> MESKKRQWALEDFEIGRPLGKGKFGNVYLAREKQSKFILALKVLFKAQLEKAGVEHQLRREVEIQSHLRHPNILRLYGYFHDATRVYLILEYAPLGTVYRELQKLSKFDEQRTATYITELAN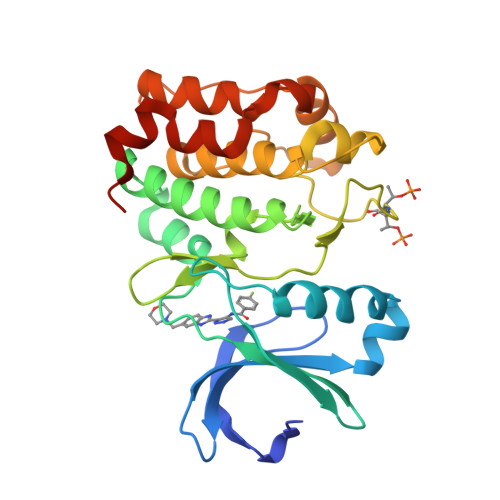ALSYCHSKRVIHRDIKPENLLLGSAGELKIADFGWSVHAPSSRRTTLCGTLDYLPPEMIEGRMHDEKVDLWSLGVLCYEFLVGKPPFEANTYQETYKRISRVEFTFPDFVTEGARDLISRLLKHNPSQRPMLREVLEHPWITANSSKHHHHHH> MAPVIPSNTDYPGPHHFEVTFQQSSTAKSATWTYSPLLKKLYCQI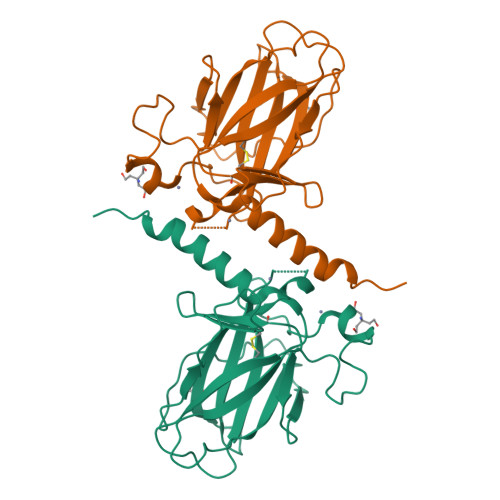AKTCPIQIKVSTPPPPGTAIRAMPVYKKAEHVTDVVKRCPNHELGRDFNEGQSAPASHLIRVEGNNLSQYVDDPVTGRQSVVVPYEPPQVGTEFTTILYNFMCNSSCVGGMNRRPILIIITLEMRDGQVLGRRSFEGRICACPGRDRKADEDHYREAENLYFQ> MTLDEEYLDITFLTENGFVRKRCPKCGKHFWTADPEREICGDPPCESYSFIGNPVFKKPFELDEMREYYLNFFERRGHGRIERYPVVARWRTDIYLTIASIADFQPFVTSGVAPPPANPLT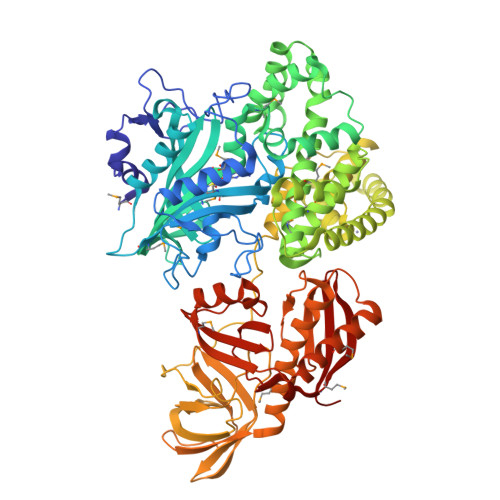ISQPCIRLDDLDSVGRTGRHLTLFEMMAHHAFNYPGKEIYWKNETVAYCTELLNELGVKKEDIVYKEEPWAGGGNAGPCLEAIVGGLEVATLVFMNLEEHPEGDIEIKGARYRKMDNYIVDTGYGLERFVWASKGTPTVYDAIFPEVVDTIIDNSNVSFNREDERVRRIVAESSKLAGIMGELRGERLNQLRKSVADTVGVSVEELEGIVVPLEKVYSLADHTRCILFMLGDGLVPSNAGAGYLARLMIRRSLRLAEELELGLDLYDLVEMHKKILGFEFDVPLSTVQEILELEKERYRTTVSKGTRLVERLVERKKKLEKDDLIELYDSHGIPVELAVGIAAEKGAEVEMPKDIYAELAKRHSKAEKVQEKKITLQNEYPATEKLYYDDPTLLEFEAEVIGVEGDFVILNRSAFYPESGGQDNDVGYLIANGGKFEVVDVLEADGVVLHVVKGAKPEVGTKVKGVIDSDVRWRHMRHHSATHVLLYSLQKVLGNHVWQAGARKEFSKARLDVTHFRRPSEEEIKEIEMLANREILANKPIKWEWMDRIEAERKFGFRLYQGGVPPGRKIRVVQVGDDVQACGGTHCRSTGEIGMLKILKVESIQDGVIRFEFAAGEA> GPATKDIPDVAGQTVDVAQKNLNVYGFTKFSQASVDSPRPAGEVTGTNPPAGTTVPVDSVIELQVSKGNQ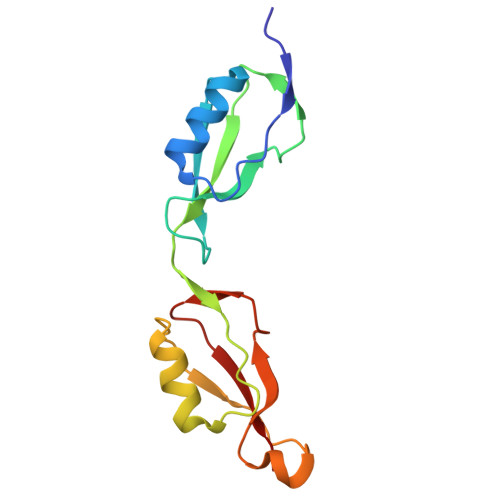FVMPDLSGMFWVDAEPRLRALGWTGMLDKGADVDAGGSQHNRVVYQNPPAGTGVNRDGIITLRFGQ>SNADPNYFIGIQFRNIPYKYDVKIPHLTFG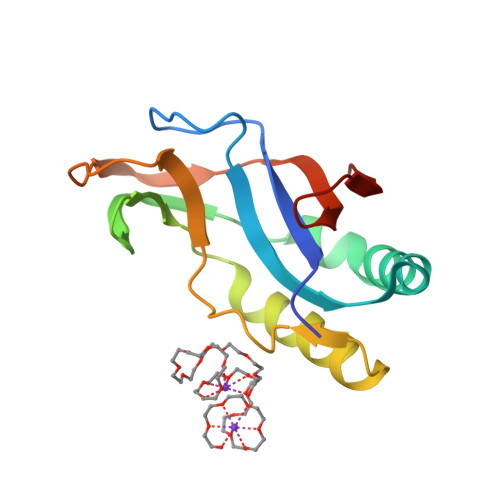VLHISDNMVPDVIDILKIMKNELFKMDITTSYTYMLSDGIYVANVSGVLSTYFKIYNVFYKNQITFGQSRMFIPHITLSFNNMRTVRIETTKLQIKSIYLRKIKGDTVFDMVE[4x]>XSLSSKDKDTVKALWGKIADKAEEIGSDALSRMLAVYPQTKTYFSHWKDLSPGSAPVNKHGKTIMGGIVDAVASIDD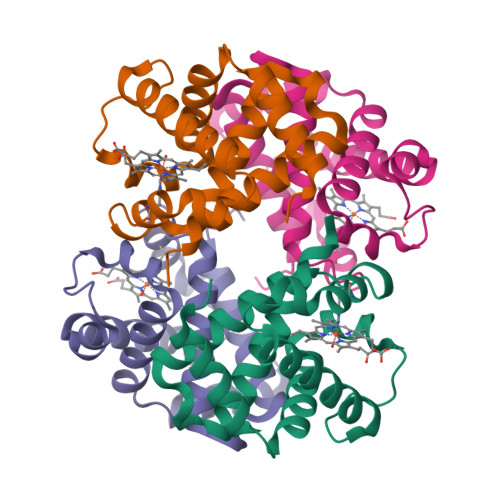LNAGLLALSELHAFTLRVDPANFKILSHCILVLLAVKFPKDFTPEVHISYDKFFSALARALAEKYR[2x];>[2x]VVWTDFERATIADIFSKLDYEAVGGATLARCLIVYPWTQRYFGNFGNLYNAAAIMGNPMIAKHGTTILHGLDRAVKNMDNIKATYAELSVLHSEKLHVDPDNFKLLSDCLTIVVAAQLGKAFSGEVQAAFQKFLSVVVSALGKQYH>[2x]HARHMLATSLV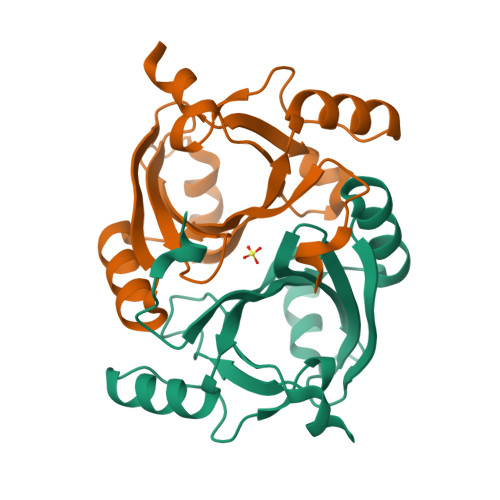TGLDHVGIAVADLDVAIEWYHDHLGMILVHEEINDDQGIREALLAVPGSAAQIQLMAPLDESSVIAKFLDKRGPGIQQLACRVSDLDAMCRRLRSQGVRLVYETARRGTANSRINFIHPKDAGGVLIELVEPAPKLAAAL> AGGHGDVGMHVKEKEKNKDENKRKDEERNKTQEEHLKEIMKHIVKIEVKGEEAVKKEAAEKLLEKVPSDVLEMYKAIGGKIYIVDGDITKHIS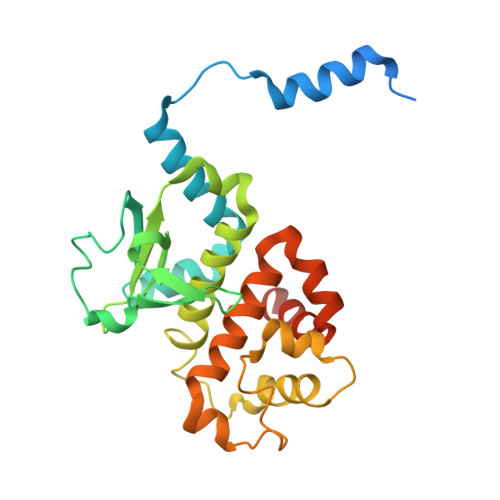LEALSEDKKKIKDIYGKDALLHEHYVYAKEGYEPVLVIQSSEDYVENTEKALNVYYEIGKILSRDILSKINQPYQKFLDVLNTIKNASDSDGQDLLFTNQLKEHPTDFSVEFLEQNSNEVQEVFAKAFAYYIEPQHRDVLQLYAPEAFNYMDKFNEQEINLSLEELKDQR> TCACACCAG;> TCTGTGA;> CTGGACA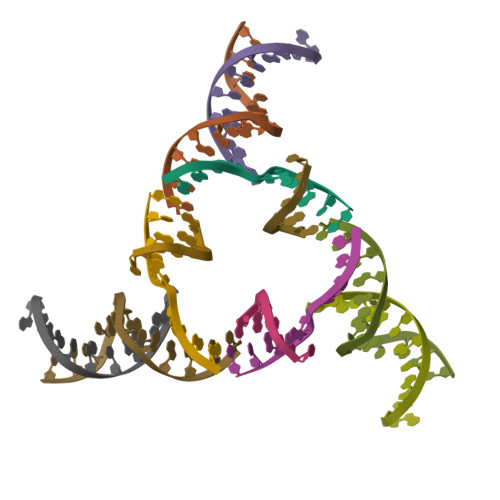CCGCATC;> GAGATGCGGTGT> MHHHHHHGGSHHWGGDPARPALGVLELKSYALGVAVADAALRAAPVELLKCEPVEPGKALIMIRGEPEAVARAMAAALETAKAGSGNLIDHAFIGRIHPALLPFLLEETAAPPIEDPDEAVLVVETKTVAAAIEAADAALDVAPVRLLRMRLSEHIGGKAYFVLAGDEEAVRKAARAVRAVAGEKLI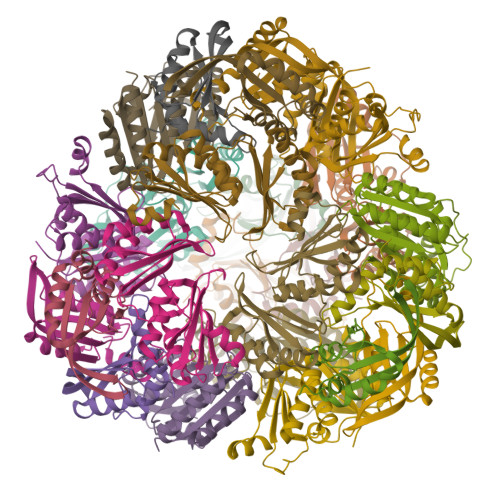DLRIIPRPHEALRGRLFF;> MPIALTVVPPEEAEPLARELVEAGLAAEVLLVPVRRIYREKGKVREEEVTLLLILVSREGVPALRAWIEARHPDDIPLFIVLAVDEEASNKRYLGYIAAETHLYSA>GSHYRPTSAYERGQRYASRLQNEFAGNISALADAENISRKIITRCINTAKLPKSVVALFSHPGELSARSGDALQKAFTDKEELLKQQASNLHEQKKAGVIFEADEVITLLTS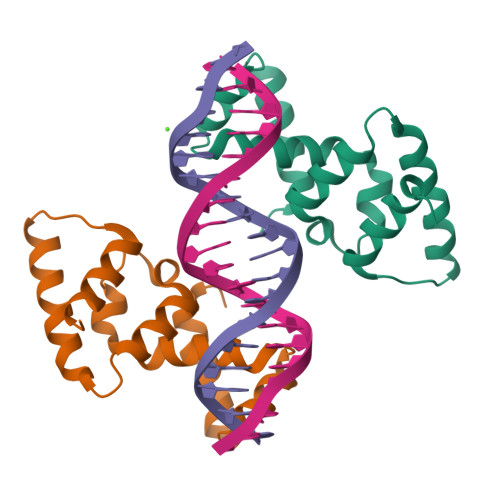VLKTSSASR[4x]> GSHMNLVIALHSYEPSHDGDLGFEKGEQLRILEQSGEWWKAQSLTTGQEGFIPFNFVAKANSLEPEPWFFKNLSRKDAERQLLAPGNTHGSFLIRESESTAGSFSLSVRDFDQNQGEVVKHYKIRNLDNGGFYISPRITFPGLHELVRHYTNASDGLC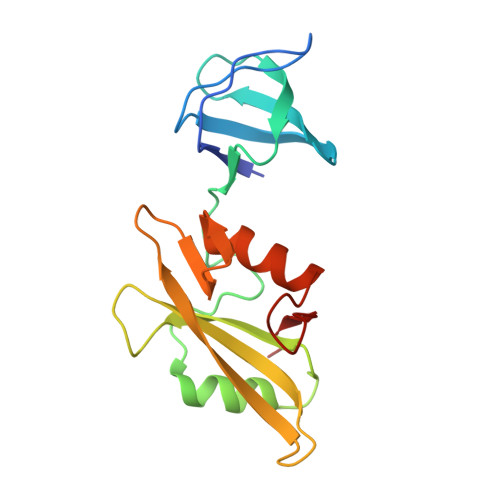TRLSRPCQT>MFHSSAMVNSHRKPMFNIHRGFYCLTAILPQICICSQFSVPSSYHFTEDPGAFPVATNGERFPWQELRLPSVVIPLHYDLFVHPNLTSLDFVASEKIEVLVSNATQFIILHSKDLEITNATLQSEEDSRYMKPGKELKVLSYPAHEQIALLVPEKLTPHLKYYVAMDFQAKLGDGFEGFYKSTYRTLGGETRILAVTDFEPTQARMAFPCFDEPLFKANFSIKIRRESRHIALSNMPKVKTIELEGGLLEDHFETTVKMSTYLVAYIVCDFHSLSGFTSSGVKVSIYASPDKRNQTHYALQASLKLLDFYEKYFDIYYPLSKLDLIAIPDFAPGAMENWGLITYRETSLLFDPKTSSASDKLWVTRVIAHELAHQWFGNLVTMEWWNDIWLNEGFAKYMELIAVNATYPELQFDDYFLNVCFEVITKDSLNSSRPISKPAETPTQIQEMFDEVSYNKGACILNMLKDFLGEEKFQKGIIQYLKKFSYRNAKNDDLWSSLSNSCLESDFTSGGVCHSDPKMTSNMLAFLGENAEVKEMMTTWTLQKGIPLLVVKQDGCSLRLQQERFLQGVFQEDPEWRALQERYLWHIPLTYSTSSSNVIHRHILKSKTDTLDLPEKTSWVKFNVDSNGYYIVHYEGHGWDQLITQLNQNHTLLRPKDRVGLIHDVFQLVGAGRLTLDKALDMTYYLQHETSSPALLEGLSYLESFYHMMDRRNISDISENLKRYLLQYFKPVIDRQSWSDKGSVWDRMLRSALLKLACDLNHAPCIQKAAELFSQWMESSGKLNIPTDVLKIVYSVGAQTTAGWNYLLEQYELSMSSAEQNKILYALSTSKHQEKLLKLIELGMEGKVIKTQNLAALLHAIARRPKGQQLAWDFVRENWTHLLKKFDLGSYDIRMIISGTTAHFS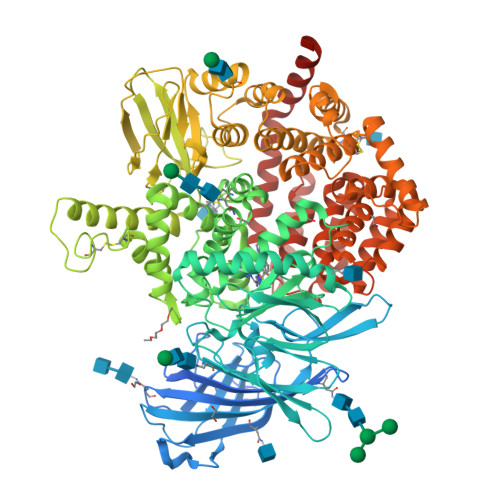SKDKLQEVKLFFESLEAQGSHLDIFQTVLETITKNIKWLEKNLPTLRTWLMVNTRHH[2x]>MQYTGKYLKKTALMLTMMAGLSAGQSQATVAPDTRSLDEIYQSALKEGGTVTVYAGGDVQSQQAGFKQAFENRFPGIKLNVIVDYSKYHDARIDNQLATDTLIPDVVQLQTVQDFPRWKKQGVLLNYKPVGWDKVYPEFRDADGAWIGAYVIAFSNLVNTQLLNEKSWPREANDYLRPDLKGNLILAYPNDDDAVLFWYKQIVDKYGWEFVEKLQEQDPVYVRGTNVPGAQITTGKYSATFTSSGALVPAAGSVTRFVLPKTDPFVSWAQRAAIFKQAKHPESAKLYLSWLLDPQTQTQVSRMWSVR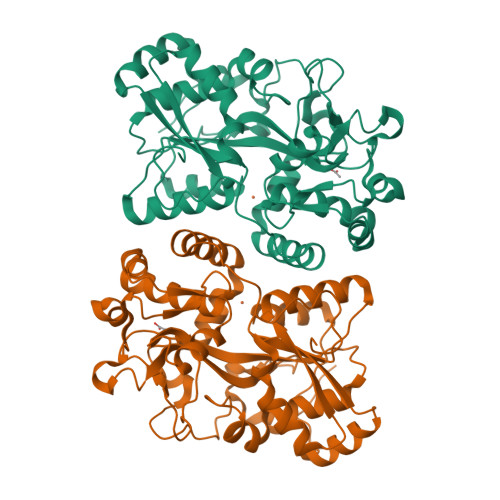TDVAPPAGYKHIWEYSNTRPQAFADFMSDRGAVERFRAQMSLYVGEAKGDPTPGWLGLHPEVPLAN[4x]> AKGRAGRSK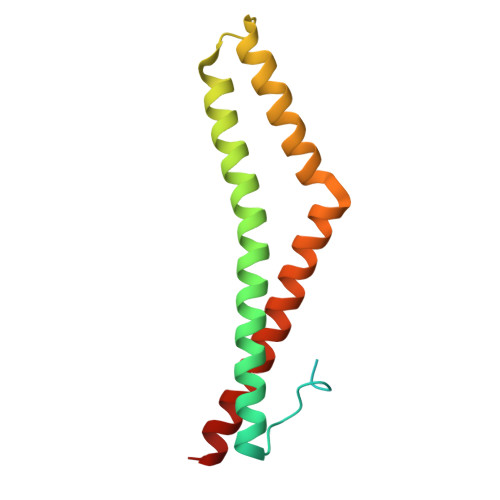RTEQDHYETDYTTGGESCDELEEDWIREYPPITSDQQRQLYKRNFDTGLQEYKSLQSVLDEINKELSRLDKELDDYREESEEYMAAADEYNRLKQVKGSADYKSKKNHCKQLKSKLSHIKKMVGDYDRQKT>MLILSFLCPAFLNAQIVTDERMFSFEEPQLPACITGVQSQLGISGAHYKDGKHSLEWTFEPNGRLELRKDLKFEKKDPTGKDLYLSAFIVWIYNEQPQDAAIEFEFLKDGRKCASFPFGINFKGWRAAWVCYERDMQGTPEEGMNELRIVAPDAKGRLFIDHLITATKVDARQQTADLQVPFVNAGTTNHWLVLYKHSLLKPDIELTPVSDKQRQEMKLLEKRFRDMIYTKGKVTEKEAETIRKKYDLYQITYKDGQVSGVPVFMVRASEAYERMIPDWDKDMLTKMGIEMRAYFDLMKRIAVAYNNSEAGSPIRKEMRRKFLAMYDHITDQGVAYGSCWGNIHHYGYSVRGLYPAYFLMKDVLREEGKLLEAERTLRWYAITNEVYPKPEGNGIDMDSFNTQTTGRIASILMMEDTPEKLQYLKSFSRWIDYGCRPAPGLAGSFKVDGGAFHHRNNYPAYAVGGLDGATNMIYLFSRTSLAVSELAHRTVKDVLLAMRFYCNKLNFPLSMSGRHPDGKGKLVPMHYAIMAIAGTPDGKGDFDKEMASAYLRLVSSDSSSAEQAPEYMPKVSNAQERKIAKRLVENGFRAEPDPQGNLSLGYGCVSVQRRENWSAVARGHSRYLWAAEHYLGHNLYGRYLAHGSLQILTAPPGQTVTPTTSGWQQEGFDWNRIPGVTSIHLPLDLLKANVLNVDTFSGMEEMLYSDEAFAGGLSQGKMN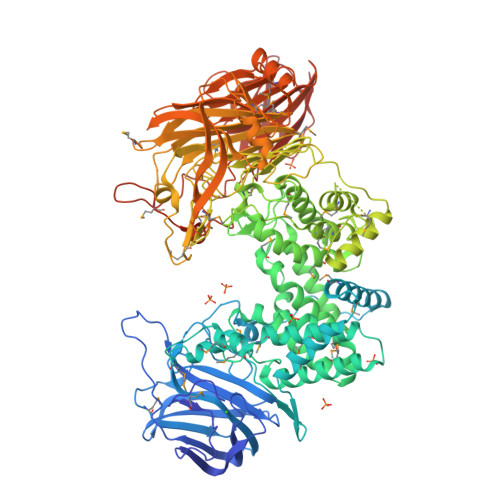GNFGMKLHEHDKYNGTHRARKSFHFIDGMIVCLGSDIENTNMDYPTETTIFQLAVTDKAAHDYWKNNAGEGKVWMDHLGTGYYVPVAARFEKNFPQYSRMQDTGKETKGDWVSLIIDHGKAPKAGSYEYAILPGTDRKTMTAFAKKPAYSVLQQDRNAHILESPSDRITSYVLFETPQSLLPGGLLQRTDTSCLVMVRKESADKVLLTVAQPDLALYRGPSDEAFDKDGKRMERSIYSRPWIDNESGEIPVTVTLKGRWKVVETPYCKVVSEDKKQTVLRFLCKDGASYEVELEKLEHHHHHH[2x]> LSQETFXD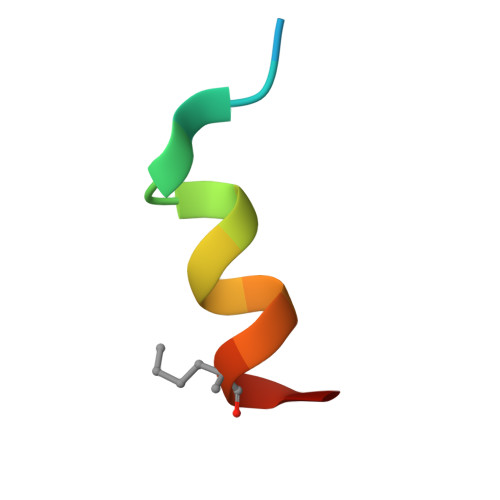LWKLLLENX The enzyme LkcE from the lankacidin polyketide biosynthetic pathway of the bacterium Streptomyces rochei represents an interesting test case for understanding such gain-of-function, as it exhibits a monoamine oxidase (MAO) protein fold yet also carries out a macrocyclization reaction. The catalytic mechanism proposed for LkcE involves initial oxidation of the amide function of LC-KA05 to an iminium ion. This is followed by attack of a C-2 enolate anion on the iminium to give the 17-membered lankacidinol A (2)8—an enzymatic intramolecular Mannich reaction.

In order to obtain complexes with LC-KA05, mutants E64A, E64Q, Y182F, R326L, and R326Q were soaked with the 1/7 substrate mixture followed by rapid acquisition of the X-ray diffraction data (owing both to the low availability of LC-KA05 and its high instability, it was not possible to carry out co-crystallization experiments). Of the five mutants, only E64Q and R326Q yielded co-complexes with 1; 7 was not observed in the active sites, as the acetate of 1 was clearly visible. The structure of the LkcE E64Q/LC-KA05 complex was solved at 3.03 Å resolution and that of the LkcE R326Q/LC-KA05 complex at 2.50 Å resolution by molecular replacement, using the structure of the LkcE/EMAA/DATD complex as the search model, and the presence of LC-KA05 confirmed using a weighted Fo−Fc omit map. LC-KA05 lies at the interface between the substrate-binding domain and the cofactor-binding domain and adopts an extended conformation. The substrate sits in a deep pocket (∼ 20 Å from the protein surface and ~ 6−8 Å wide), and is surrounded by hydrophobic residues (L70, Y168, Y182, L185, M189, W200, L324, F345, V396, and G398). In addition to these hydrophobic interactions, binding is likely mediated by seven hydrogen bonds: two to the lactone ring at the entry point of the pocket (by N179 and T397), one to the acetate at C-7 by the side chain of Q428, and four to the lactoyl moiety (two with Y168, and one each with E64 and R326). Notably, in this configuration, the lactoyl portion of LC-KA05 stacks against the FAD isoalloxazine in a position appropriate for hydride transfer (the amide proton is situated at 3.2 Å from the FAD N-5). On the other hand, superposition of the R326Q/LC-KA05 structure and that of the holo wild type shows that if LC-KA05 bound into the wild type in the same orientation as in the LkcE R326Q/LC-KA05 complex, its C-24 hydroxyl would sterically clash with R326. Indeed, the fact that the R326Q mutant retains essentially wild-type activity means that we have not simply captured a non-productive complex with the enzyme. Taken together, these data are consistent with residues E64 and R326 playing critical roles in the catalytic mechanism (although R can be substituted by Q without a significant effect on activity), whereas Y182 is not essential.

>[2x]GPGSMTVVEAKSRIAVVGGGGSGSVAAWLLARRHDVTLFEADEYLGGHAYSHPVETDQGTLHVDMGVEHFNEKLSPNLFRLLTDFGIGTYVAPSSVHVDFPGEQQSWNNLDFLGELREELHEEFDRFHQEMNQLPTSGDDSYKQMSIGEYLDKHGYSKSFKYKAMNPILSIYSGCHAPSLDYNLMYVALSFSMNLLSFFSAGYWRKAQGGIHSYLARIESDLGERVRLNTPVEAVVPTQSGVTVLAGGQEHHFDQVVFATHADVTLRLLRTSDQQYRDLLGDFAYVPVESVLHQDESWLSPAGGGAYCQFRMPEGFELARAEEQMGSLTQNCNVLHPYRKVSSPILITFDPQEDVDPERVIVRREWKLPQLRPVDVRRKKRLHEIQGLNGLWFCGTDTSVTGHEGAIVSGMVIADRLGVPHPFPDDAPAAAQFRGIKEFMGV[(1S,2R)-2-(2-hydroxybenzene-1-carbonyl)cyclopentyl]acetic acid 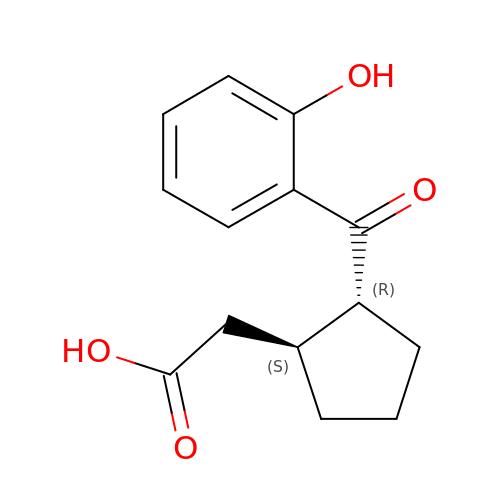| C14 H16 O4 | LULBZYDRYZGRST-VHSXEESVSA-N>EQEQQYDVHGNVISAAVYQKFHVYGPEDMVFDGDAGGLTIPGAGAFWGTLFTSDLQRLYKDTVSFQYNALGTYLNINFFDSSGGFLGHIQAGAVSAVVGVGGGSGSWHNWEVA[2x]

Virulence-associated proteins (Vaps) contribute to the virulence of the pathogen Rhodococcus equi, but their mode of action has remained elusive. All Vaps share a conserved core of about 105 amino acids that folds into a compact eight-stranded antiparallel β-barrel with a unique topology. At the top of the barrel, four loops connect the eight β-strands. The same applies to virulence-associated protein B (VapB), which is also encoded on a virulence plasmid; this plasmid is mostly absent from foal isolates and is predominantly found in porcine R. equi isolates.

Here, we determined the structure of the protease-resistant VapB core in a new crystal form with two molecules in the asymmetric unit. The crystals diffracted to 1.71 Å resolution and the structure was solved by molecular replacement. The same three residues (Asn152, Asn159 and Asn161) from both chains contribute to nitrate binding. In one of them, the loop regions at the top of the barrel adopt a different conformation from other Vap structures. An all-against-all analysis of the available Vap structures using the DALI server revealed that with regard to these loops, chain A of our new VapB structure is most distant from the other Vap structures. Okoko and coworkers suggested that Vap proteins may have functions that only manifest upon the conformational changes that frequently accompany the binding of small molecules to proteins. Our new VapB structure reveals that despite the crossover connections, VapB can form a large cavity between the β3–β4 loop and the β7–β8 loop. The bottom of the large VapB cavity is formed by hydrophobic residues (Val96, Phe105, Phe130, Ala153, Leu158 and Ala177), while its side and mouth contain both hydrophobic (for example Ile124 and Val181) and polar (for example Ser98, Gln103, Thr123, Tyr151 and Ser179) residues. The large cavity in VapB contains 12 ordered water molecules (A311, A314, A320, A322, A332, A344, A357, A360, A380, A390, A401 and A403), giving a hint on the size and shape of a putative ligand.> DAKNIKKGPAPFYPLEDGTAGEQLHKAMKRYALVPGTIAFTDAHIEVNITYAEYFEMSVRLAEAMKRYGLNTNHRIVVCSENSLQFFMPVLGALFIGVAVAPANDIYNERELLNSMNISQPTVVFVSKKGLQKILNVQKKLPIIQKIIIMDSKTDYQGFQSMYTFVTSHLPPGFNEYDFVPESFDRDKTIALIMNSSGSTGLPKGVALPHRTACVRFSHARDPIFGNQIIPDTAILSVVPFHHGFGMFTTLGYLICGFRVVLMYRFEEELFLRSLQDYKIQSALLVPTLFSFFAKSTLIDKYDLSNLHEIASGGAP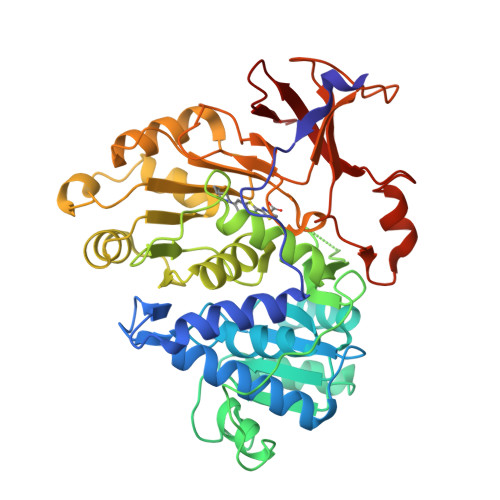LSKEVGEAVAKRFHLPGIRQGYGLTETTSAILITPEGDDKPGAVGKVVPFFEAKVVDLDTGKTLGVNQRGELCVRGPMIMSGYVNNPEATNALIDKDGWLHSGDIAYWDEDEHFFIVDRL> MSNFTPDACNVDSGLDSVLPPSLYALVFTLGLPANLLALWAAWLQVRKGRELGVYLLNLSLSDLLLICALPPWTDYYLRRDVWGYGPGACRLFGFVFYTNLYVGAAFLSCVSADRYLAVAHPLRFPGARPIRSAAAVSALIWMLELAANAPPLLGEAIHRDRYNHTFCYESYPLSGRGAALANVGRVLAGFLLPWGVMMLCYAGLLRALRGSASCEQRERRR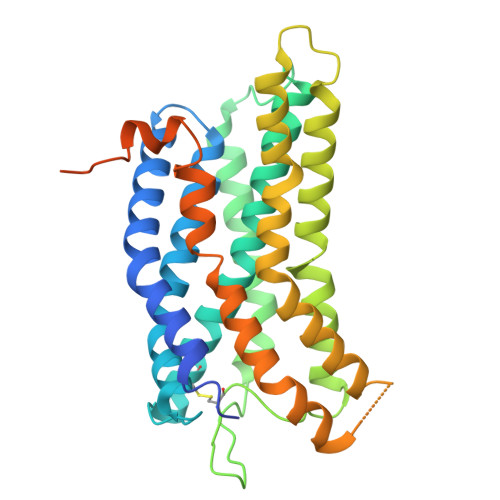VRRLALGLPCVALLCYGPYHALLLLRSLVFLVGGGSVDAGGGCALEERLFPAYHASLALATLNCLADPALYCLACPGARGEVAKVVGGVVAWAMGKERRAWGERGGNGRGCGEGEEVGMVELRGNGREFVV>[4x]MARIIVVTSGKGGVGKTTSSAAIATGLAQKGKKTVVIDFAIGLRNLDLIMGCERRVVYDFVNVIQGDATLNQALIKDKRTENLYILPASQTRDKDALTREGVAKVLDDLKAMDFEFIVCDS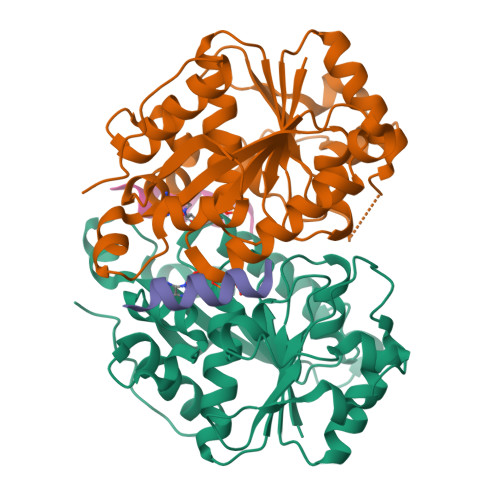PAGIETGALMALYFADEAIITTNPEVSSVRDSDRILGILASKSRRAENGEEPIKEHLLLTRYNPGRVSRGDMLSMEDVLEILRIKLVGVIPEDQSVLRASNQGEPVILDINADAGKAYADTVERLLGEERPFRFIEEEK;>KNTANIAKERLQIIVAERRR[4x]>[2x]MVQKESQATLEERESELSSNPAASAGASLEPPAAPAPGEDNPAGAGGAA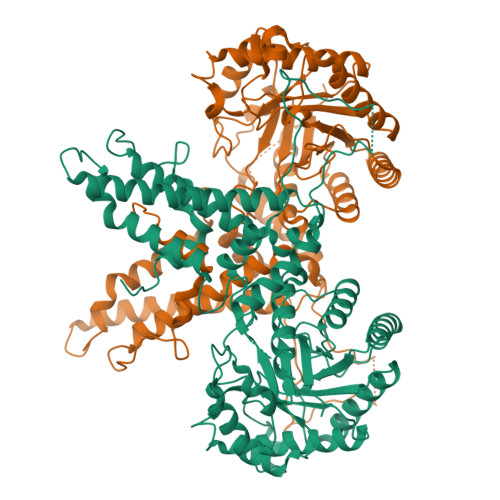VAGAAGGARRFLCGVVEGFYGRPWVMEQRKELFRRLQKWELNTYLYAPKDDYKHRMFWREMYSVEEAEQLMTLISAAREYEIEFIYAISPGLDITFSNPKEVSTLKRKLDQVSQFGCRSFALLFDDIDHNMCAADKEVFSSFAHAQVSITNEIYQYLGEPETFLFCPTEYCGTFCYPNVSQSPYLRTVGEKLLPGIEVLWTGPKVVSKEIPVESIEEVSKIIKRAPVIWDNIHANDYDQKRLFLGPYKGRSTELIPRLKGVLTNPNCEFEANYVAIHTLATWYKSNMNGVRKDVVMTDSEDSTVSIQIKLENEGSDEDIETDVLYSPQMALKLALTEWLQEFGVPHQYSSRQVAHSGAKASVVDGTPLVAAPSLNATTVVTTVYQEPIMSQGAALSGEPTTLTKEEEKKQPDEEPMDMVVEKQEETDHKNDNQILSEIVEAKMAEELKPMDTDKESIAESKSPEMSMQEDCISDIAPMQTDEQTNKEQFVPGPNEKPLYTAEPVTLEDLQLLADLFYLPYEHGPKGAQMLREFQWLRANSSVVSVNCKGKDSEKIEEWRSRAAKFEEMCGLVMGMFTRLSNCANRTILYDMYSYVWDIKSIMSMVKSFVQWLGCRSHSSAQFLIGDQEPWAFRGGLAGEFQRLLPIDGANDLFFQPPPLTPTSKVYTIRPYFPKDEASVYKICREMYDDGVGLPFQSQPDLIGDKLVGGLLSLSLDYCFVLEDEDGICGYALGTVDVTPFIKKCKISWIPFMQEKYTKPNGDKELSEAEKIMLSFHEEQEVLPETFLANFPSLIKMDIHKKVTDPSVAKSMMACLLSSLKANGSRGAFCEVRPDDKRILEFYSKLGCFEIAKMEGFPKDVVILGRSL> MAHHHHHHSSGLEVLFQGPEDITDIPKLADYLKLFRPKKLMLKA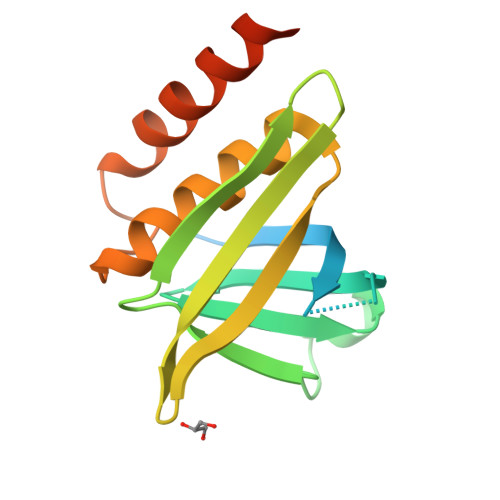CKQYWFVFKDTSIAYFKNKELEQGEPIEKLNLRGCEIVPDVNVSGRKFGIKLLIPVADGMNEVYLRCDHEDQYARWMAACILASKGKTMADSSYQPEVISILSFLKMKNRNSSPLVASSLE> MPEEALIVVDMQRDFMPGGALPVPEGDKIIPKVNEYIRKFKEKGALIVATR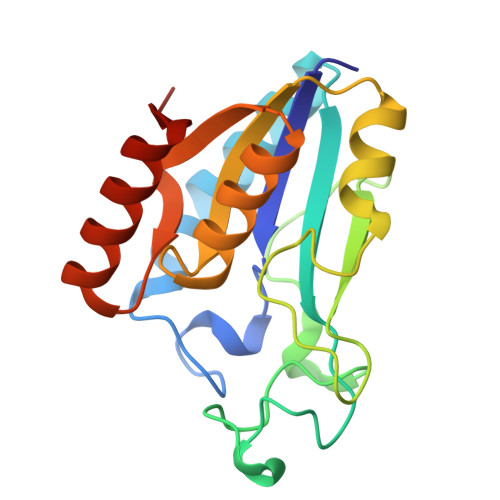DWHPENHISFRERGGPWPRHCVQNTPGAEFVVDLPEDAVIISKATEPDKEAYSGFEGTDLAKILRGNGVKRVYICGVATEYCVRATALDALKHGFEVYLLRDAVKGIKPEDEERALEEMKSRGIKIVQF> MAHHHHHHEPAYQRPDAPMPSAYPNGPAYATPGAPRANPGEPAAAELGWRNFLADAQLQQLVALALANNRDLRVATLDIDEARALYRIQRAAQFPAIDASVGLTSQRMSPALRAPGQSAAINSYDASVGLTHFEIDLFGRVRSLSHAAQEQYLATEEARRSVHISLVAEVANTYLTLLADRALLALAQDTLRSQQDAADMIHRGKQAGAMAQLDEHRADTQVQTARVAAEQYTRQIAQDENALAVLIGGPLPAGVSRAAPLGDRALLAEFPAGLPSTLLERRPDIMAAEHRLIAANAQIGAARAAFFPRITLTGALGVASASLAGLFSGGVAWLFVPQLTLPIFNA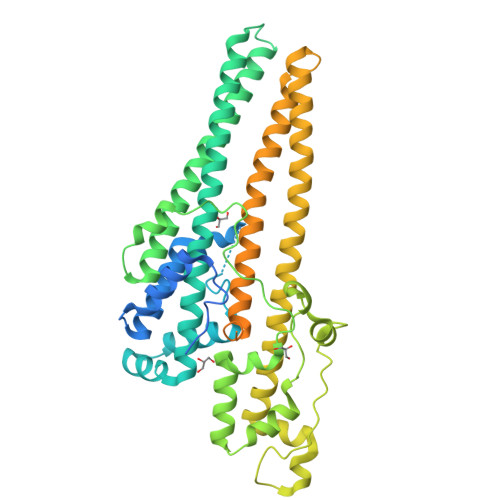GSNQANLDLATVRRDINVAGYEHTIQDAFREVADNLAARATYEREVKAQEAMIRDLAETKRLADMRFRNGVDDYFGVFDAQRQLFAAQQLLVTYKLAGLTSRVTLYKALGGGWVESAGAAAAQPRTGQAAPMARPAATPPQTTRPAPVARSQTVPPRTVQPPIAQPATAQPQTAQAAPVAQSQTIPLRTVQPPIAQSSTSQPQTAQAAPITQARTTPLRTAQPPAARQQAPQSAPAAQPEAVPPQTAQPPIFQP> GVPGALSNQP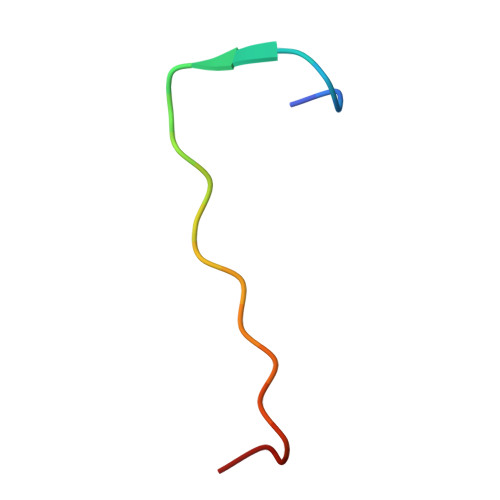APPNEAPIATP> MTIGIDKINFYVPKYYVDMAKLAEARQVDPNKFLIGIGQTEMAVSPVNQDIVSMGANAAKDIITDEDKKKIGMVIVATESAVDAAKAAAVQIHNLLGIQPFARCFEMKEACYAATPAIQLAKDYLATRPNEKVLVIATDTARYGLNSGGEPTQGAGAVAMVIAHNPSILALNEDAVAYTEDVYDFWRPTGHKYPLVDGALSKDAYIRSFQQSWNEYAKRQGKSLADFASLCFHVPFTKMGKKALESIIDNADETTQERLRSGYEDAVDYNRYVGNIYTGSLYLSLISLLENRDLQAGETIGLFSYGSGSVVEFYSATLVEGYKDHL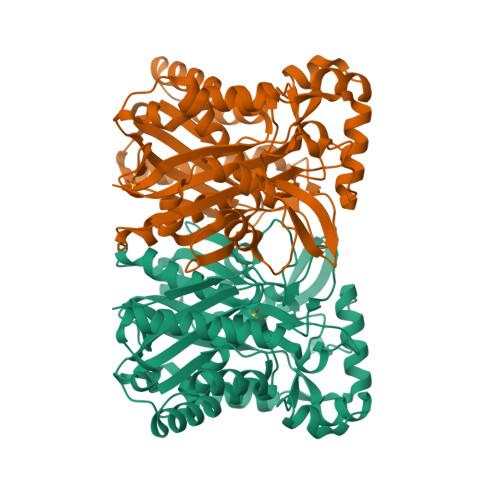DQAAHKALLNNRTEVSVDAYETFFKRFDDVEFDEEQDAVHEDRHIFYLSNIENNVREYHRPE> MSDNRRRRREEDDSDSENELPPSSPQQHFRGGMNPVSSPIGSPDMINPEGDDNEVDDVPDIDEVEEQMNEVDLMDDNMYEDYAADHNRDRYDPDQVDDREQQELSLSERRRIDAQLNERDRLLRNVAYIDDEDEEQEGAAQLDEMGLPVQRRRRRRQYEDLENSDDDLLSDMDIDPLREELTLESLSNVKANSYSEWITQPNVSRTIARELKSFLLEYTDETGRSVYGARIRTLGEMNSESLEVNYRHLAESKAILALFLAKCPEEMLKIFDLVAMEATELHYPDYARIHSEIHVRISDFPTIYSLRELRESNLSSLVRVTGVVTRRTGVFPQLKYVKFNCLKCGSILGPFFQDSNEEIRISFCTNCKSKGPFRVNGEKTVYRNYQRVTLQEAPGTVPPGRLPRHREVILLADLVDVSKPGEEVEVTGIYKNNYDGNLNAKNGFPVFATIIEANSIKRREGNTANEGEEGLDVFSWTEEEEREFRKISRDRGIIDKIISSMAPSIYGHRDIKTAVACSLFGGVPKNVNGKHSIRGDINVLLLGDPGTAKSQILKYVEKTAHRAVFATGQGASAVGLTASVRKDPITKEWTLEGGALVLADKGVCLIDEF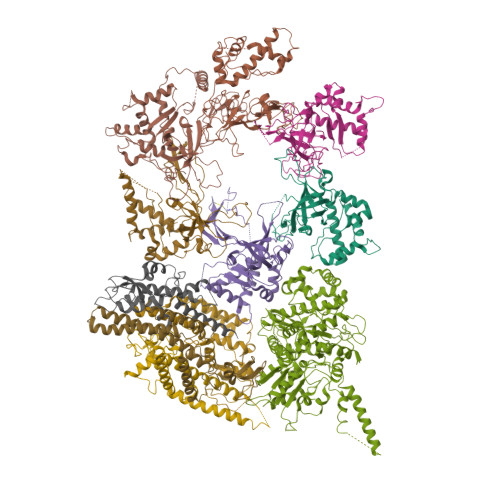DKMNDQDRTSIHEAMEQQSISISKAGIVTTLQARCSIIAAANPNGGRYNSTLPLAQNVSLTEPILSRFDILCVVRDLVDEEADERLATFVVDSHVRSHPENDEDREGEELKNNGESAIEQGEDEINEQLNARQRRLQRQRKKEEEISPIPQELLMKYIHYARTKIYPKLHQMDMDKVSRVYADLRRESISTGSFPITVRHLESILRIAESFAKMRLSEFVSSYDLDRAIKVVVDSFVDAQKVSVRRQLRRSFAIYTLGH;> MEGSTGFDGDATTFFAPDAVFGDRVRRFQEFLDTFTSYRDSVRSIQVYNSNNAANYNDDQDDADERDLLGDDDGDDLEKEKKAASSTSLNILPHRIIISLDDLREFDRSFWSGILVEPAYFIPPAEKALTDLADSMDDVPHPNASAVSSRHPWKLSFKGSFGAHALSPRTLTAQHLNKLVSVEGIVTKTSLVRPKLIRSVHYAAKTGRFHYRDYTDATTTLTTRIPTPAIYPTEDTEGNKLTTEYGYSTFIDHQRITVQEMPEMAPAGQLPRSIDVILDDDLVDKTKPGDRVNVVGVFKSLGAGGMNQSNSNTLIGFKTLILGNTVYPLHARSTGVAARQMLTDFDIRNINKLSKKKDIFDILSQSLAPSIYGHDHIKKAILLMLMGGVEKNLENGSHLRGDINILMVGDPSTAKSQLLRFVLNTASLAIATTGRGSSGVGLTAAVTTDRETGERRLEAGAMVLADRGVVCIDEFDKMTDVDRVAIHEVMEQQTVTIAKAGIHTTLNARCSVIAAANPVFGQYDVNRDPHQNIALPDSLLSRFDLLFVVTDDINEIRDRSISEHVLRTHRYLPPGYLEGEPVRERLNLSLAVGEDADINPEEHSNSGAGVENEGEDDEDHVFEKFNPLLQAGAKLAKNKGNYNGTEIPKLVTIPFLRKYVQYAKERVIPQLTQEAINVIVKNYTDLRNDDNTKKSPITARTLETLIRLATAHAKVRLSKTVNKVDAKVAANLLRFALLGEDIGNDIDEEESEYEEALSKRSPQKSPKKRQRVRQPASNSGSPIKSTPRRSTASSVNATPSSARRILRFQDDEQNAGEDDNDIMSPLPADEEAELQRRLQLGLRVSPRRREHLHAPEEGSSGPLTEVGTPRLPNVSSAGQDDEQQQSVISFDNVEPGTISTGRLSLISGIIARLMQTEIFEEESYPVASLFERINEELPEEEKFSAQEYLAGLKIMSDRNNLMVADDKVWRV;> MSQQSSSPTKEDNNSSSPVVPNPDSVPPQLSSPALFYSSSSSQGDIYGRNNSQNLSQGEGNIRAAIGSSPLNFPSSSQRQNSDVFQSQGRQGRIRSSASASGRSRYHSDLRSDRALPTSSSSLGRNGQNRVHMRRNDIHTSDLSSPRRIVDFDTRSGVNTLDTSSSSAPPSEASEPLRIIWGTNVSIQECTTNFRNFLMSFKYKFRKILDEREEFINNTTDEELYYIKQLNEMRELGTSNLNLDARNLLAYKQTEDLYHQLLNYPQEVISIMDQTIKDCMVSLIVDNNLDYDLDEIETKFYKVRPYNVGSCKGMRELNPNDIDKLINLKGLVLRSTPVIPDMKVAFFKCNVCDHTMAVEIDRGVIQEPARCERIDCNEPNSMSLIHNRCSFADKQVIKLQETPDFVPDGQTPHSISLCVYDELVDSCRAGDRIEVTGTFRSIPIRANSRQRVLKSLYKTYVDVVHVKKVSDKRLDVDTSTIEQELMQNKVDHNEVEEVRQITDQDLAKIREVAAREDLYSLLARSIAPSIYELEDVKKGILLQLFGGTNKTFTKGGRYRGDINILLCGDPSTSKSQILQYVHKITPRGVYTSGKGSSAVGLTAYITRDVDTKQLVLESGALVLSDGGVCCIDEFDKMSDSTRSVLHEVMEQQTISIAKAGIITTLNARSSILASANPIGSRYNPNLPVTENIDLPPPLLSRFDLVYLVLDKVDEKNDRELAKHLTNLYLEDKPEHISQDDVLPVEFLTMYISYAKEHIHPIITEAAKTELVRAYVGMRKMGDDSRSDEKRITATTRQLESMIRLAEAHAKMKLKNVVELEDVQEAVRLIRSAIKDYATDPKTGKIDMNLVQTGKSVIQRKLQEDLSREIMNVLKDQASDSMSFNELIKQINEHSQDRVESSDIQEALSRLQQEDKVIVLGEGVRRSVRLNNRV;> MSFDRPEIYSAPVLQGESPNDDDNTEIIKSFKNFILEFRLDSQFIYRDQLRNNILVKNYSLTVNMEHLIGYNEDIYKKLSDEPSDIIPLFETAITQVAKRISILSRAQSANNNDKDPENTSMDTDSLLLNSLPTFQLILNSNANQIPLRDLDSEHVSKIVRLSGIIISTSVLSSRATYLSIMCRNCRHTTSITINNFNSITGNTVSLPRSCLSTIESESSMANESNIGDESTKKNCGPDPYIIIHESSKFIDQQFLKLQEIPELVPVGEMPRNLTMTCDRYLTNKVIPGTRVTIVGIYSIYNSKNGAGSGRSGGGNGGSGVAIRTPYIKILGIQSDVETSSIWNSVTMFTEEEEEEFLQLSRNPKLYEILTNSIAPSIFGNEDIKKAIVCLLMGGSKKILPDGMRLRGDINVLLLGDPGTAKSQLLKFVEKVSPIAVYTSGKGSSAAGLTASVQRDPMTREFYLEGGAMVLADGGVVCIDEFDKMRDEDRVAIHEAMEQQTISIAKAGITTVLNSRTSVLAAANPIYGRYDDLKSPGDNIDFQTTILSRFDMIFIVKDDHNEERDISIANHVINIHTGNANAMQNQQEENGSEISIEKMKRYITYCRLKCAPRLSPQAAEKLSSNFVTIRKQLLINELESTERSSIPITIRQLEAIIRITESLAKLELSPIAQERHVDEAIRLFQASTMDAASQDPIGGLNQASGTSLSEIRRFEQELKRRLPIGWSTSYQTLRREFVDTHRFSQLALDKALYALEKHETIQLRHQGQNIYRSGV;> MSSPFPADTPSSNRPSNSSPPPSSIGAGFGSSSGLDSQIGSRLHFPSSSQPHVSNSQTGPFVNDSTQFSSQRLQTDGSATNDMEGNEPARSFKSRALNHVKKVDDVTGEKVREAFEQFLEDFSVQSTDTGEVEKVYRAQIEFMKIYDLNTIYIDYQHLSMRENGALAMAISEQYYRFLPFLQKGLRRVVRKYAPELLNTSDSLKRSEGDEGQADEDEQQDDDMNGSSLPRDSGSSAAPGNGTSAMATRSITTSTSPEQTERVFQISFFNLPTVHRIRDIRSEKIGSLLSISGTVTRTSEVRPELYKASFTCDMCRAIVDNVEQSFKYTEPTFCPNPSCENRAFWTLNVTRSRFLDWQKVRIQENANEIPTGSMPRTLDVILRGDSVERAKPGDRCKFTGVEIVVPDVTQLGLPGVKPSSTLDTRGISKTTEGLNSGVTGLRSLGVRDLTYKISFLACHVISIGSNIGASSPDANSNNRETELQMAANLQANNVYQDNERDQEVFLNSLSSDEINELKEMVKDEHIYDKLVRSIAPAVFGHEAVKKGILLQMLGGVHKSTVEGIKLRGDINICVVGDPSTSKSQFLKYVVGFAPRSVYTSGKASSAAGLTAAVVRDEEGGDYTIEAGALMLADNGICCIDEFDKMDISDQVAIHEAMEQQTISIAKAGIHATLNARTSILAAANPVGGRYNRKLSLRGNLNMTAPIMSRFDLFFVILDDCNEKIDTELASHIVDLHMKRDEAIEPPFSAEQLRRYIKYARTFKPILTKEARSYLVEKYKELRKDDAQGFSRSSYRITVRQLESMIRLSEAIARANCVDEITPSFIAEAYDLLRQSIIRVDVDDVEMDEEFDNIESQSHAASGNNDDNDDGTGSGVITSEPPADIEEGQSEATARPGTSEKKKTTVTYDKYVSMMNMIVRKIAEVDREGAEELTAVDIVDWYLLQKENDLGSLAEYWEERRLAFKVIKRLVKDRILMEIHGTRHNLRDLENEENENNKTVYVIHPNCEVLDQLEPQDSS;> MSAALPSIQLPVDYNNLFNEITDFLVTFKQDTLSSDATRNENEDENLDAENIEQHLLEKGPKYMAMLQKVANRELNSVIIDLDDILQYQNEKFLQGTQADDLVSAIQQNANHFTELFCRAIDNNMPLPTKEIDYKDDVLDVILNQRRLRNERMLSDRTNEIRSENLMDTTMDPPSSMNDALREVVEDETELFPPNLTRRYFLYFKPLSQNCARRYRKKAISSKPLSVRQIKGDFLGQLITVRGIITRVSDVKPAVEVIAYTCDQCGYEVFQEVNSRTFTPLSECTSEECSQNQTKGQLFMSTRASKFSAFQECKIQELSQQVPVGHIPRSLNIHVNGTLVRSLSPGDIVDVTGIFLPAPYTGFKALKAGLLTETYLEAQFVRQHKKKFASFSLTSDVEERVMELITSGDVYNRLAKSIAPEIYGNLDVKKALLLLLVGGVDKRVGDGMKIRGDINVCLMGDPGVAKSQLLKAICKISPRGVYTTGKGSSGVGLTAAVMKDPVTDEMILEGGALVLADNGICCIDEFDKMDESDRTAIHEVMEQQTISISKAGINTTLNARTSILAAANPLYGRYNPRLSPLDNINLPAALLSRFDILFLMLDIPSRDDDEKLAEHVTYVHMHNKQPDLDFTPVEPSKMREYIAYAKTKRPVMSEAVNDYVVQAYIRLRQDSKREMDSKFSFGQATPRTLLGIIRLSQALAKLRLADMVDIDDVEEALRLVRVSKESLYQETNKSKEDESPTTKIFTIIKKMLQETGKNTLSYENIVKTVRLRGFTMLQLSNCIQEYSYLNVWHLINEGNTLKFVDDGTMDTDQEDSLVSTPKLAPQTTASANVSAQDSDIDLQDA;> MYGDLGNKLVLEAKRTKQLYARSNQDVNLPMYHEDIIRNILKEVSNLRKNTEYLKEQQQLGMLDDKVAKCQYFVTLLCMERNKRCLLAYQRLRTDILDSMAWNNNGLDLMSSITFSQQDTNNLSHQEQEYLKEYCDLITDLKSGDLVDIDLSGSLVPPSDVFIDVRVLKDAGEIQTEYGVFNLIKDSQFFVRQSDVERLIQQGYLQKI;> MSLPAHLQQTFSPEEIQFIVENEPIKIFPRITTRQKIRGDDRGTGNHTRWQLITTDDKALNNMVAMRSTEVVLWIALLLKQQSKCSIVAPQWLTTKELDRKIQYEKTHPDRFSELPWNWLVLARILFNKAKDDFHDPIHELRGKIQDLREIRQIKVLKGLKYLNESHLQLDNLSLLEINELRPFITEIMDKLREIHTASLTAGTENDEEEFNI;> MGYYDIDDVLADGTEFPCKFQYDIPGLGYLENNPGRPITKNTKLSLPLWLARILAIVGGDEALVDEEPVPFVELLPPDMFSTKVMNAIKTDPVALDLHSINSHFFSLAIKWIMLFSEKELANVVSELLLQRAQELNHHASSLSIDLNADSTGKNSANTNIATSTFLLKLEEMEKEIYKKSHESYKDTKRWMFKK;> MDINIDDILAELDKETTAVDSTKITQGSSSTTHRDANTIVGSSLDLNDKTQIYVSPQQDFSDLMKSWKNERCSPELLPYPHQLMKRLLNRISMQSQLIENISMGFLDMQNASNANPPMPNESKLPLLCMETELERLKFVIRSYIRCRLSKIDKFSLYLRQLNEDENSLISLTDLLSKDEIKYHDTHSLIWLKLVNDSILKYMPEELQAINDTEGSVNMIDEPDWNKFVFIHVNGPPDGKWNEDPLLQENEFGKPCYTVTIPDLKEEVELTIGSIYVMRYEVIRDLLRDDKVALI;> MYYGISQFSEAYNKILRNSSSHSSCQLVIFVSCLNIDALCATKMLSLLFKKQLVQSQIVPIFGYSELRRHYSQLDDNINSLLLVGFGGVIDLEAFLEIDPQEYVIDTDEKSGEQSFRRDIYVLDAHRPWNLDNIFGSQIIQCFDDGTVDDTLGEQKEAYYKLLELDEESGDDELSGDENDNNGGDDEATDADEVTDEDEEDEDETISNKRGNSSIGPNDLSKRKQRKKQIHEYEGVLEEYYSQGTTVVNSISAQIYSLLSAIGETNLSNLWLNILGTTSLDIAYAQVYNRLYPLLQDEVKRLTPSSRNSVKTPDTLTLNIQPDYYLFLLRHSSLYDSFYYSNYVNAKLSLWNENGKKRLHKMFARMGIPLSTAQETWLYMDHSIKRELGIIFDKNLDRYGLQDIIRDGFVRTLGYRGSISASEFVEALTALLEVGNSTDKDSVKINNDNNDDTDGEEEEDNSAQKLTNLRKRWVSNFWLSWDALDDRKVELLNRGIQLAQDLQRAIFNTGVAILEKKLIKHLRIYRLCVLQDGPDLDLYRNPLTLLRLGNWLIECCAESEDKQLLPMVLASIDENTDTYLVAGLTPRYPRGLDTIHTKKPILNNFSMAFQQITAETDAKVRIDNFESSIIEIRREDLSPFLEKLTLSGLLDYKDHDGDYKDHDIDYKDDDDK3-(4-Tert-butylphenyl)-5-(1H-pyrazol-4-yl)furo[3,2-b]pyridine | 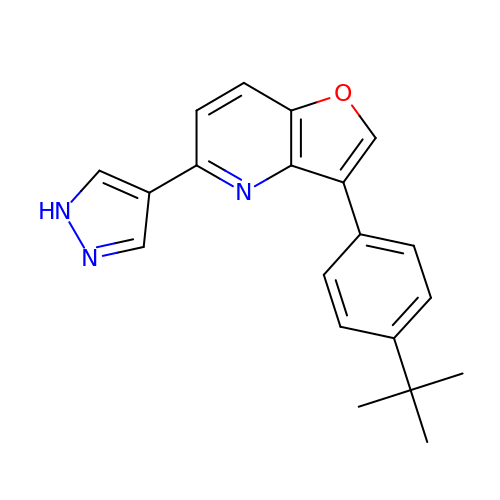C20 H19 N3 O | OOLXXVMFVSTNLJ-UHFFFAOYSA-N>[2x]MEALKIALLGGGTVGSAFYNLVLERAEELSAFGVVPRFLGVLVRDPRKPRAIPQELLRAEPFDLLEADLVVEAMGGVEAPL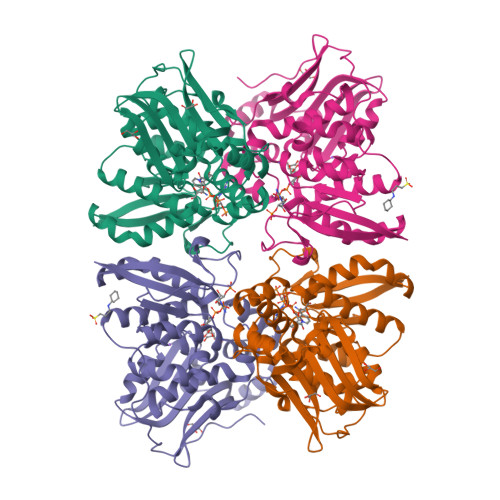RLVLPALEAGIPLITANKALLAEAWESLRPFAEEGLIYHEASVMAGTPALSFLETLRGSELLELHGILNGTTLYILQEMEKGRTYAEALLEAQRLGYAEADPTLDVEGIDAAHKLTLLARLLVDPGFPFAEVEAQGIARLTPEVLQKAEARGERVRLVASLFGEGGRWRAAVAPRRLPQDHPLARARGNALWVRARPLGEAFVTGPGAGGGATASGLFADLLRFLSGAPGHLPAPRARPPLEEGSPWPGVE>[4x]MASWSHPQFEKGAGTMIVIFVHGWSVTHTNTYGELPQWLENQSKQGKLDIQVGNIYLGRYISFDDTVTVDDIARAFDQAVRDEIADKLRDGQRFACITHSTGGPIVRKWMDLYFKNNLAKCPLSHLIMLAPANHGSALAQLGKSRLGRIKSFFEGIEPGKCVLDWLELGSDMSWQLNESWLDYDCTANGVYSFVLTGQ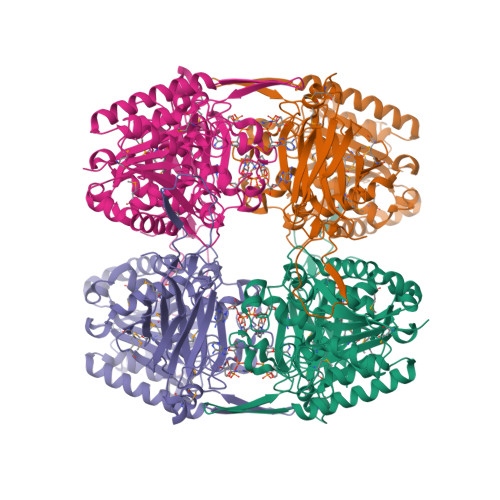KIDRQFYDAVNSYTGESGSNGVVRVAATNMNYSLLKLHQEGDNGESLVVAKMTRTQPMAFGVLPGLSHSGKNIGIIRSITMANAATHPTAIWILRCLQVKSRDSYNKLVKELDNITKETQKNEHKEFVKTLVFTREYITNRYSMIIFRLIDDRGNHLIDYDLYLTAGPQYSEQALPAGFFVDRQRNLNNRGKLTYFLDYDIMEGGINTPKMQGNLGFRVKAYPESSDQALAYYRLLDFHSSLADIHKILHPNETVMVEIMLQRRVDRTVFRISNNLTPAKISGKPTGKKID> MNIFRLTGDLSHLAAIIILLLKIWKSRSCAGISGKSQLLFALVFTTRYLDLFTSFISLYNTSMKLIYIACSYATV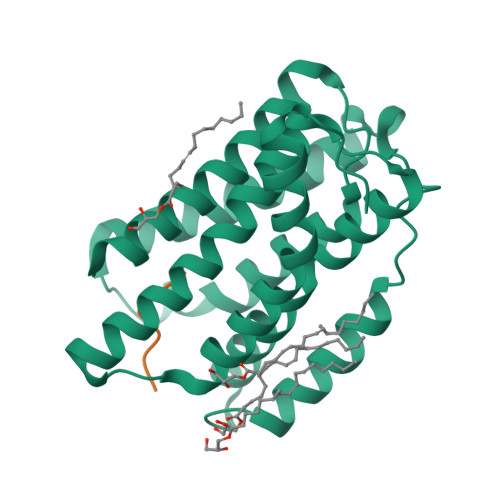YLIYMKFKATYDGNHDTFRVEFLIVPVGGLSFLVNHDFSPLEILWTFSIYLESVAILPQLFMISKTGEAETITTHYLFFLGLYRALYLVNWIWRYYFEGFFDLIAVVAGVVQTVLYCDFFYLYVTKVLKGKKLSLPA;> TAEHDEF>[2x]VTSEAYVSGMLFCLGIFLSFYLLTVLLACWENWRQKKKTLLVAIDRACPESGHPRVLADSFPGSSPYEGYNYGSFENVDTLTDIDSDKNVIRTKQYLYVADLARKDKRVLRKKYQIYFWNIATIAVFYALPVVQLVITYQTVVNVTGNQDICYYNFLCAHPLGNLSAFNNILSNLGYILLGLLFLLIILQREINHNRALLRNDLCALECGIPKHFGLFYAMGTALMMEGLLSACYHVCPNYTNFQFDTSFMYMIAGLCMLKLYQKRHPDINASAYSAYACLAIVIFFSVLGVVFGKGNTAFWIVFSIIHIIATLLLSTQLYYMGRWKLDSGIFRRILHVLYTDCIRQCSGPLYVDRMVLLVMGNVINWSLAAYGLIMRPNDFASYLLAIGICNLLLYFAFYIIMKLRSGERIKLIPLLCIVCTSVVWGFALFFFFQGLSTWQKTPAESREHNRDCILLDFFDDHDIWHFLSSIAMFGSFLVLLTLDDDLDTVQRDKIYVFDYKDHDGDYKDHDIDYKDDDDK

Human SIDT1 and SIDT2 are closely related members of the SID-1 transmembrane family, and have been implicated in various biological processes such as glucose and lipid metabolism, innate immunity, and tumorigenesis. Here, we present the cryo-electron microscopy (cryo-EM) structures of human SIDT1 and SIDT2. Both structures reveal an overall architecture of a dimeric arrangement composed of an extracellular domain (ECD) rich in β-strands and a transmembrane domain (TMD) with 11 passes, highlighting the remarkable structural congruence. Importantly, the ECDs of SIDT1 and SIDT2 bind synthetic plant-derived miRNA only under acidic conditions.

The TMDs of both proteins consist of 11 transmembrane helices and feature two pairs of conserved disulfide bonds that are essential for structural integrity. Notably, both SIDT1 and SIDT2 exhibit a potential zinc-binding site with three histidine residues within TMDs, which is responsible for lipid hydrolytic activity. Regarding the TMD, while the overall arrangement is similar in both SIDT1 and SIDT2, different transmembrane helices (TMs) contribute to dimerization. In contrast, SIDT2 relies more on interactions between TM2 and TM6 for dimerization. The electron density maps exhibited well-defined main-chain connectivity and side-chain densities in the ECDs, while the TMDs have relatively lower quality and resolution. Overall, while the ECD structure exhibits consistency, the individual helices of the TMD in SID-1 transmembrane family members show flexibility, highlighting the dynamic nature of these proteins in performing specific functions in membranes.>GSGSTRDYEIQRERIELGRCIGEGQFGDVHQGIYMSPENPALAVAIKTCKNCTSDSVREKFLQEALTMRQFDHPHIVKLIGVITENPVWIIMELCTLGELRSFLQVRKYSLDLASLILYAYQLSTALAYLESKRFVHRDIAARNVLVSSNDCVKLGDFGLSRYMEDSTYYKASKGKLPIKWMAPESINFRRFTSASDVWMFGVCMWEILMHGVKPFQGVKNNDVIGRIENGERLPMPPNCPPTL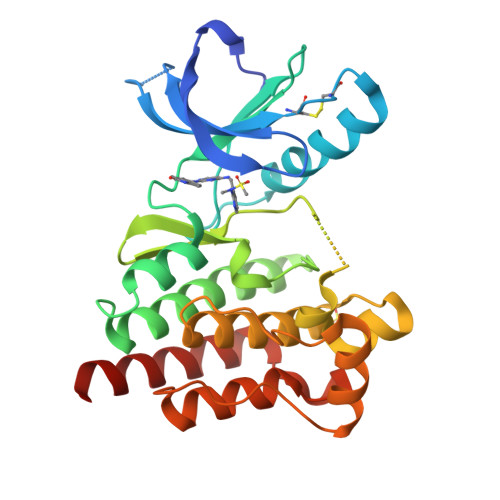YSLMTKCWAYDPSRRPRFTELKAQLSTILEEEKAQQEE[2x]> GPLGSEKIEKDNAFAFDLLQTTRKHVTEANVFISPLSVSMALNMTLNGAAGVTADEMKTALRETGYTMEDINEYSHSLREALLKVDPSTTIGMANSIWYKQGELVKEPFILANRTHYDAEVKAVDFSSPATLPAINGWCAQKTNDKITKILDYIPGNAFMYLINAVYFKGIWVTQFKKSDTKRAPFRKADGTTQEVNMMAQKSTFGYTTDECCQYLEMDYGNKAFSMIVMLPNEGQTTRDVIEQLDNKHWSMIIKGIRPTQVSLRMPRFKTECKYGLEKKILPEMGMNVPFTETADFPGITDAAIFISRVIHKTFVQVD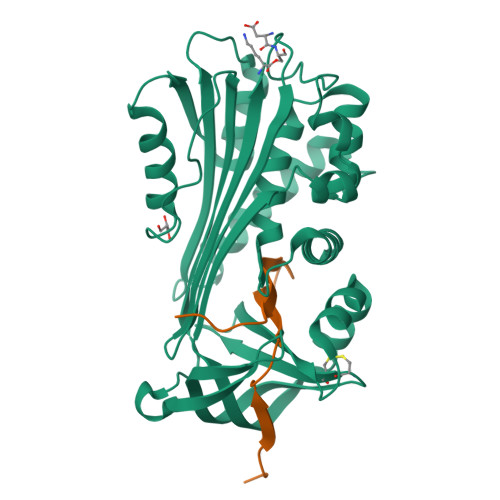EEGTEAAAVTAVEMVK;> TSSPSTTPINFHINKPFVFAIREKSTGVILFIGEIGEVKE[6-methyl-4-[[(5-methyl-2-oxidanylidene-furan-3-ylidene)amino]methyl]-5-oxidanyl-pyridin-3-yl]methyl dihydrogen phosphate | C13 H15 N2 O7 P | 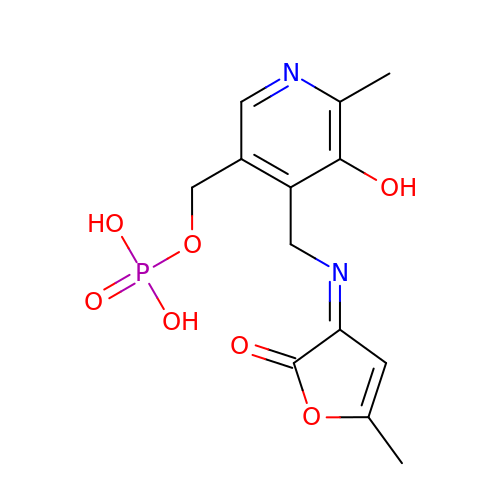SDTUNOOKUCGPLI-RVDMUPIBSA-N Chromatin remodeling complex NoRC (nucleolar remodeling complex) interacts with the rDNA promoter regions of silent genes repressing rDNA transcription. It consists of TIP5 (TTF-I interacting protein 5), also known as BAZ2A (bromodomain [BRD] adjacent to zinc finger domain protein 2A), which is the largest subunit, and the adenosine triphosphatase (ATPase) SNF2h (sucrose nonfermenting protein 2 homologue). BAZ2B shares 29% sequence identity with TIP5 at the full-length level and harbors similar domain organization. Both proteins contain a MBD (methyl-CpG-binding domain), also known as TAM (TTF-IIP5, ARBP, MeCP1) domain, AT-hook DNA-binding domains, DDT (DNA binding homeobox and different transcription factors), and a PHD (plant homeodomain) zinc finger adjacent to a BRD at their C terminus. Our crystal structures combined with biophysical and mutagenesis data demonstrate that PHD zinc fingers recognize N-terminal unmodified H3K4 tail, whereas the TIP5 and BAZ2B BRDs recognize H4K16ac and H3K14ac, respectively, with specificity pattern KacXXR.

A peptide soak of unmodified H3 histone to apo crystals allowed us to determine the peptide-binding at high resolution (1.91 Å). The structure of the complex revealed that the N terminus of H3 is recognized by main chain hydrogen-bond interactions with backbone carbonyl groups of P1714, E1715, and G1716 located in loop 2 and by hydrophobic interaction of the side chain of H3A1, which was well accommodated in a hydrophobic pocket formed by L1692 and P1714. Peptide binding was associated with structural changes in loop 2, which was shifted about 2 Å in the peptide bound state. As observed in other PHD finger complexes, the H3 peptide binds to the surface in an antiparallel β sheet conformation with the TIP5 β1 stabilized by backbone hydrogen bonds with residues L1693, L1691, and D1688. An important feature of the structure is the recognition of the H3K4 side chain, in which the N terminus and loop1 of the TIP5 PHD finger harbor the lysine side chain, forming a shallow but well-defined groove. The H3K4 epsilon amino group interacts through hydrogen bonds with two main chain carbonyl oxygens (V1677, G1685) and a long-range salt bridge (4.2 Å) with D1688 located in the TIP5 310 helix. The limited space in the lysine binding cavity and the absence of the typical aromatic cage present in methyl-lysine interacting PHD domains restricts binding of this PHD finger to unmodified lysine side chains. A comparison of available structures of PHD fingers in complex with H3K4me0 highlights how the lysine side chain recognition is essentially formed by acidic residues and interactions through carbonyl backbone groups. Structural details of this interaction confirm the absence of an aromatic cage and the presence of negatively charged residues that form hydrogen bonds with the K4 side chain.

>[4x]HMSVNKVTCLVCRKGDNDEFLLLCDGCDRGCHIYCHRPKMEAVPEGDWFCTVCLAQQV;>[3x]ARTKQ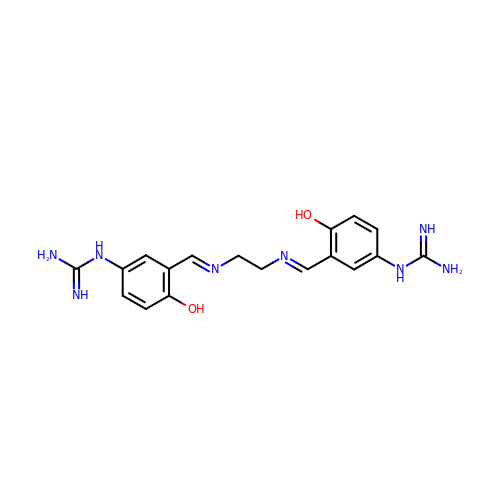N,N'''-{ethane-1,2-diylbis[nitrilo(E)methylylidene(4-hydroxybenzene-3,1-diyl)]}diguanidine | C18 H22 N8 O2 | VDYARAMMHWMLLR-WDBPGAOMSA-N> GG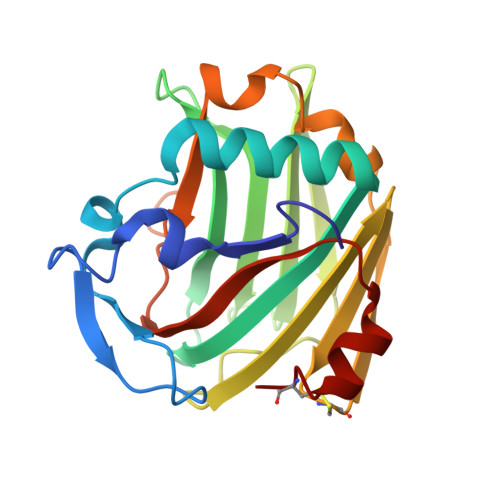DNSVFDIFELTGAARKGSGRRLVKGPDPSSPAFRIEDANLIPPVPDDKFQDLVDAVRTEKGFLLLASLRQMKKTRGTLLALERKDHSGQVFSVVSNGKAGTLDLSLTVQGKQHVVSVEEALLATGQWKSITLFVQEDRAQLYIDCEKMENAELDVPIQSVFTRDLASIARLRIAKGGVNDNFQGVLQNVRFVFGTTPEDILRNKGCS>[2x]GGSRRILLPKNVIVECMVATHHNSRNASIWLGCGHTDRGQLSFLDLNTEGYTSEEVADSRILCLALVHLPVEKESWIVSGTQSGTLLVINTEDGKKRHTLEKMTDSVTCLYCNSFSKQSKQKNFLLVGTADGKLAIFEDKTVKL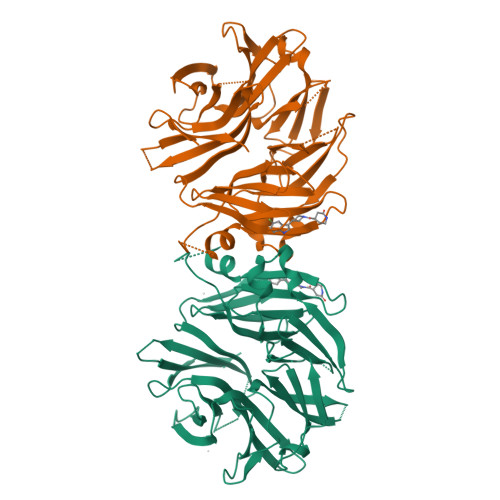KGAAPLKILNIGNVSTPLMCLSESTNSTERNVMWGGCGTKIFSFSNDFTIQKLIETRTSQLFSYAAFSDSNIITVVVDTALYIAKQNSPVVEVWDKKTEKLCGLIDCVHFLREVTVKENKESKHKMSYSGRVKTLCLQKNTALWIGTGGGHILLLDLSTRRLIRVIYNFCNSVRVMMTAQLGSLKNVMLVLGYNRKNTEGTQKQKEIQSCLTVWDINLPHEVQNLEKHIEVRKELAEKMRRTSVE Herein, Moesziomyces aphidis DSM 70725 aromatic dioxygenase (MapADO) is characterized through X-ray crystallography, biophysical as well as biochemical assays, substrate docking and mutagenesis. MapADO features a seven-bladed β-propeller fold and a Fe2+ center coordinated by four histidine residues and shares a conserved structural motif with homologous enzymes despite low sequence identity (<38%). Similar proteins were termed aromatic dioxygenase (ADO), , apocarotenoid or alkene cleaving oxygenase (ACO). These enzymes primarily act on aromatic compounds with a hydroxy group in 4-position and use a mononuclear Fe2+ iron that is embraced by four histidines. O2 is activated by this nonheme iron and reacts with the C–C double bond of a substrate, eventually leading to C–C bond scission and two carbonyl species as the reaction products.

Acetate bound in product-free crystals formed hydrophobic interactions (L41, F340), indicating stable but nonspecific coordination. By analyzing the protein structure both in its native form and in complexes with vanillin 1, 4-hydroxybenzaldehyde (HBA, 3), and ortho-vanillin 5, we uncover the nuances of ligand binding and coordination within MapADO’s active site. MapADO features a seven-bladed β-propeller fold with an Fe2+ ion at the active site coordinated by H200, H251, H316, and H510. Fe2+ is coordinated to H200, H251, H316, and H510 and a water molecule. The sixth coordination site is occluded by T156. Although MapADO presents two molecules in the asymmetric unit, biophysical analyses suggest it is monomeric in solution: It eluted at 9.6 mL upon size exclusion chromatography on a Superdex 75 10/300 GL column, indicating a protein size of ca. 60 kDa which is consistent with its theoretical molecular weight (62.8 kDa). MapADO’s catalytic pocket lacks a conventional substrate access tunnel. Instead, it features a confined cavity closed by three Phe side chains, unlike other CCO structures with tunnels leading to the catalytic Fe.

>[2x]MWSHPQFEKAPTATQEPVPVPVTSKAAPSHGYVHPTDILPSGWPTATDLSGGAQPRRFEGTIFDVMTRGTIPKELHGTFYRIMPDYAQPPTYYKGGELNAPIDGDGTVAAFRFKDGKVDYRQRFVETDRFKVERRARKSMYGLYRNPYTHHPCVRQTVESTANTNVVMHAGRFLAMKENGNAYEMDPHTLKTLGYNPFNLPSKTMTAHPKQCSVTGNLVGFGYEAKGLATKDVYYFEVDPSGKVVRDLWLEAPWCAFIHDCALTPNYLVLMLWPFEANLERMKAGGHHWAYDYTKPITWITIPRGAKSKDEVKYWHWKNGMPIHTASGFEDEQGRIIIDSSLVHGNAFPFFPPDSDEQKKKQEADGTPKAQFVRWTIDPRKDNNEQLPDPEVILDTPSEFPQIDNRFMGVEYSSAFINVFVPDRSDGNKNVFQGLNGLAHYKRKEGTTEWYYAGDNCLIQEPVFSPRSKDAPEGDGFVLAIVDRLDLNRSEVVVIDTRDFTKAVAAVQLPFAIRSGIHGQWIPGEVTPDFETKGLVDLPKEEHWAPLSQSPYDPDA> MGSSHHHHHHSSGENLYFQGHMTQQPQAKYRHDYRAPDYQITDIDLTFDLDAQKTVVTAVSQAVRHGASDAPLRLNGEDLKLVSVHINDEPWTAWKEEEGALVISNLPERFTLKIINEISPAANTALEGLYQSGDALCTQCQAEGFRHITYYLDRPDVLARFTTKIIADKIKYPFLLSNGNRVAQGELENGRHWVQWQDPFPKPCYLFALVAGDFDVLRDTFTTRSGREVALELYVDRGNLDRAPWAMTSLKNSMKWDEERFGLEYDLDIYMIVAVDFFNMGAMENKGLNIFNSKYVLARTDTATDKDYLDIERVIGHEYFHNWTGNRVTCRDWFQLSLKEGLTVFRDQEFSSDLGSRAVNRINNVRTMRGLQFAEDASPMAHPIRPDMVIEMNNFYTLTVYEKGAEVIRMIHTLLGEENFQKGMQLYFERHDGSAATCDDFVQAMEDASNVDLSHFRRWYSQSGTPIVTVKDDYNPETEQYTLTISQR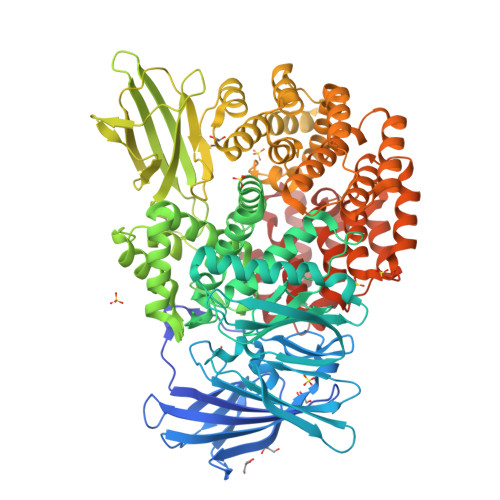TPATPDQAEKQPLHIPFAIELYDNEGKVIPLQKGGHPVNSVLNVTQAEQTFVFDNVYFQPVPALLCEFSAPVKLEYKWSDQQLTFLMRHARNDFSRWDAAQSLLATYIKLNVARHQQGQPLSLPVHVADAFRAVLLDEKIDPALAAEILTLPSVNEMAELFDIIDPIAIAEVREALTRTLATELADELLAIYNANYQSEYRVEHEDIAKRTLRNACLRFLAFGETHLADVLVSKQFHEANNMTDALAALSAAVAAQLPCRDALMQEYDDKWHQNGLVMDKWFILQATSPAANVLETVRGLLQHRSFTMSNPNRIRSLIGAFAGSNPAAFHAEDGSGYLFLVEMLTDLNSRNPQVASRLIEPLIRLKRYDAKRQEKMRAALEQLKGLENLSGDLYEKITKALA>MSTKKKPLTQEQLEDARRLKAIYEKKKNELGLSQESVADKMGMGQSGVGALFNGINALNAYNAALLAKILKVSVEEFSPSIAREIYEMYEAVSDAKRIEGFTLSEEILKSDKQLSVDAQFFTKPLTDGMAIRSEGKIYFVDKQASL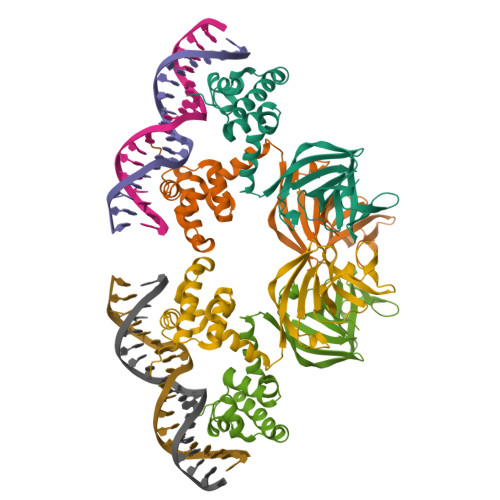SDGLWLVDIEGAISIRELTKLPGRKLHVAGGKVPFECGIDDIKTLGRVVGVYSEVNLVPRGSHHHHHH[2x]>LTCVKSNSIWFPTSEDCPDGQNLCFKRWQYISPRMYDFTRGCAATCP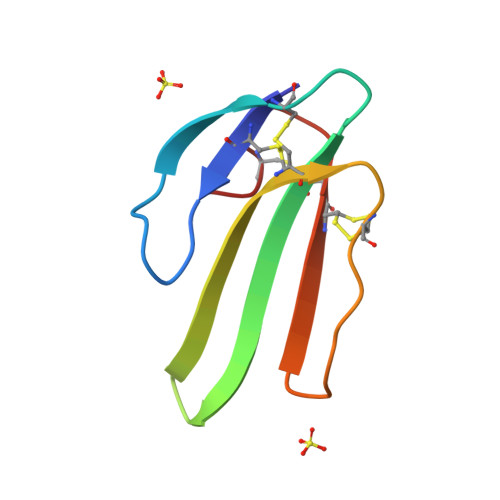KPTNVRETIRCCGTDKCNK[2x]>[12x]SNAMNSQLTLRALERGDLRFIHNLNNNRNIMSYWFEEPYESFDELEELYNKHIHDNAERRFVVEDAQKNLIGLVELIEINYIHRSAEFQIIIAPEHQGKGFAR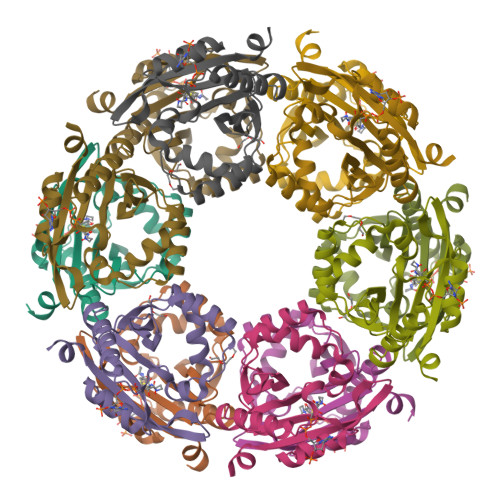TLINRALDYSFTILNLHKIYLHVAVENPKAVHLYEECGFVEEGHLVEEFFINGRYQDVKRMYILQSKYLNRSE>[2x]MASSASGLRRGHPAGGEENMTETDAFYKREMFDPAEKYKMDHRRRGIALIFNHERFFWHLTLPERRGTCADRDNLTRRFSDLGFEVKCFNDLKAEELLLKIHEVSTVSHTDADCFVCVFLSHGEGNHIYAYDAKIEIQTLTGLFKGDKCHSLVGKPKIFIIQACRGNQHDVPVIPLDVVDNQTEKLDTNITEVDAASVYTLPAGADFLMCYSVAEGYYSHRETVNGSWYIQDLCEMLGKYGSSLEFTELLTLVNRKVSQRRVDFCKDPSAIGKKQVPCFASMLTKKLHFFPKSNLEHHHHHH

Caspases belong to a highly conserved family of cysteine proteases that have essential roles in programmed cell death, inflammation, differentiation, neuronal development and axon pruning. In addition to being activated by initiator and effector caspases, Casp6 can be activated by a unique intramolecular self-cleavage mechanism due to its longer intersubunit linker. Excess neuronal active Casp6 is associated with Alzheimer disease (AD) neuropathology and age-dependent cognitive impairment. By investigating the activity of four rare natural Casp6 variants (Casp6-A34E, Casp6-E35K, Casp6-A109T, and Casp6-T182S) and employing X-ray crystallography along with molecular modelling, we have identified a putative allosteric pocket on mature active Casp6.

Following our previous work, which described rare natural Casp6-R65W and Casp6-G66R variants with significantly impaired activity, we examined four additional missense rare variants with single amino acid substitutions located remotely from Casp6 active site: Casp6-A34E, Casp6-E35K, Casp6-A109T, and Casp6-T182S. A34, E35, A109, and T182 are not conserved in 12 human caspases and in Casp6 from different species. To assess the effect of mutations on Casp6 structure and function, we solved apo mature crystal structures of Casp6-E35K and Casp6-A109T but crystallisation attempts were not successful for the two other Casp6 variants. Casp6 variants were catalytically active against Ac-VEID-AFC but Casp6-A34E, Casp6-E35K, and Casp6-T182S, displayed lower activity than Casp6-WT in enzyme concentration-dependent manner whereas the activity of Casp6-A109T was comparable to Casp6-WT. Casp6-A34E, Casp6-A109T, and Casp6-T182S did not show significant changes in kinetic parameters, KM, and kcat, for Ac-VEID-AFC hydrolysis compared with Casp6-WT, whereas Casp6-E35K displayed slightly reduced kcat and consequently showed ~2-fold reduced catalytic efficiency kcat/KM. In addition, E35K substitution disrupts a salt bridge between E35 from the large subunit and K284 from the small subunit of the same Casp6-WT protomer, possibly further destabilising a functional oligomeric state of Casp6. The Casp6-A109T crystal structure did not reveal any significant changes around the mutation site, supporting our findings that A109T substitution does not have a significant impact on Casp6 activity.> SDKIIHLTDDSFDTDVLKADGAILVDFWAEWCGPCKMIAPILDEIADEYQGKLTVAKLNIDQNPGTAPKYGIRGIPTLLLFKNGEVAATKVGALSKGQLKEFL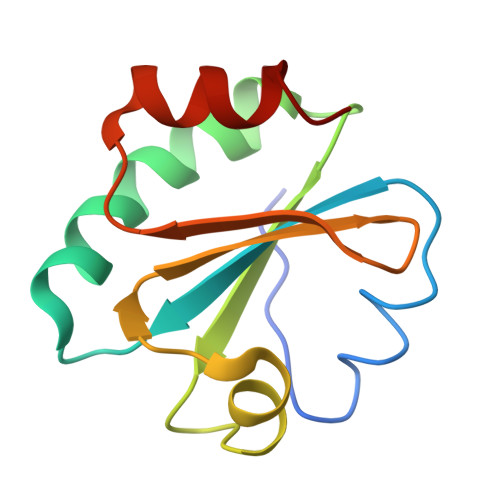DANLA> 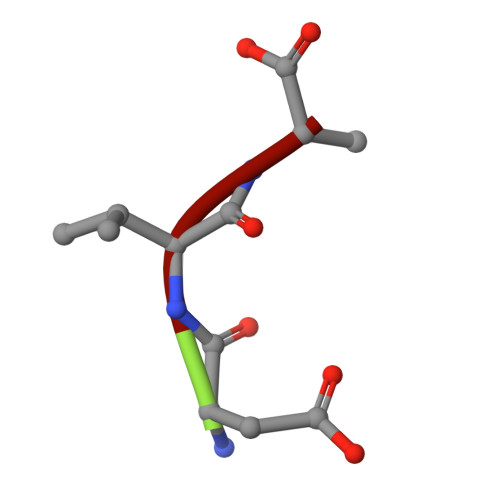DVA> QPCPCPGGSSCAIVPKTKEVVCTHCPTGTAGKRCELCDDGYFGDP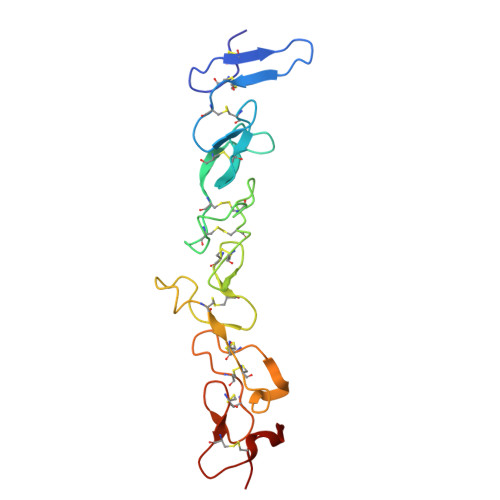LGSNGPVRLCRPCQCNDNIDPNAVGNCNRLTGECLKCIYNTAGFYCDRCKEGFFGNPLAPNPADKCKACACNPYGTVQQQSSCNPVTGQCQCLPHVSGRDCGTCDPGYYNLQSGQGCER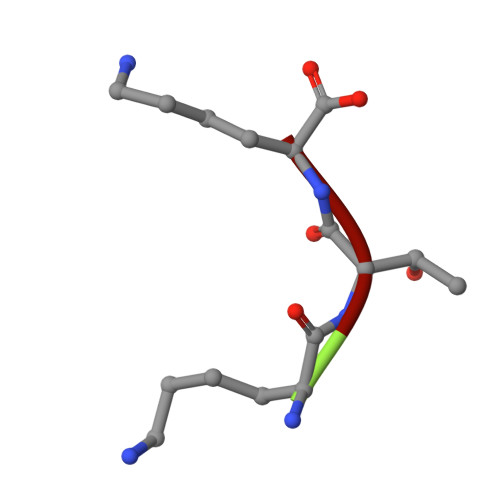> KTK> MNNQPQGTNSVPNSIGNIFSNIGTPSFNMAQIPQQLYQSLTPQQLQMIQQRHQQLLRSRLQQQQQQQQQTSPPPQTHQSPPPPPQQSQPIANQSATSTPPPPPAPHNLHPQIGQVPLAPAPINLPPQIAQLPLATQQQVLNKLRQQAIAKNNPQVVNAITVAQQQVQRQIEQQKGQQTAQTQLEQQRQLLVQQQQQQQLRNQIQRQQQQQFRHHVQIQQQQQKQQQQQQQHQQQQQQQQQQQQQQQQQQQQQQQQQQQQQQQQQQQQQGQIPQSQQVPQVRSMSGQPPTNVQPTIGQLPQLPKLNLPKYQTIQYDPPETKLPYPTYWSDKKADTDTLLYEQIIQRDKINKYSLIRETNGYDPFSIYGFSNKEYISRLWHTLKYYQDLKNTRMKSITSTSQKIPSASIW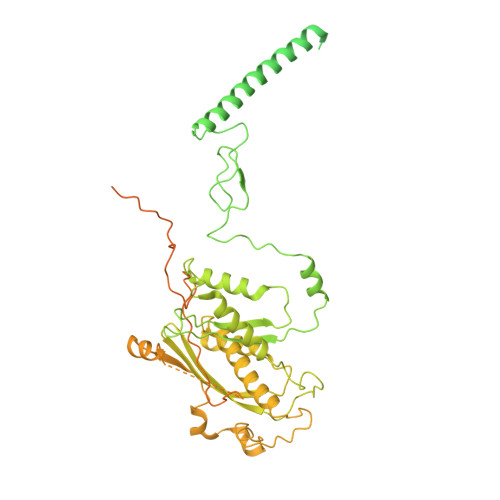GNGYSGYGNGITNTTTRVIPQVEVGNRKHYLEDKLKVYKQAMNETSEQLVPIRLEFDQDRDRFFLRDTLLWNKNDKLIKIEDFVDDMLRDYRFEDATREQHIDTICQSIQEQIQEFQGNPYIELNQDRLGGDDLRIRIKLDIVVGQNQLIDQFEWDISNSDNCPEEFAESMCQELELPGEFVTAIAHSIREQVHMYHKSLALLGYNFDGSAIEDDDIRSRMLPTITLDDVYRPAAESKIFTPNLLQISAAELERLDKDKDRDTRRKRRQGRSNRRGMLALSGTSASNTSMNGVHNTVAAGNASSLPPGEILLPDIADIPRTFRTPVPSTLMPGGVDVGPSVESYELRNTTTYKSRPDRPKPVSPPCYIIDHIPGHSLLLSIKLPGKVNTKEEFAAAPNDTSSGTNAMLPSPESLKTKLNSNIRAGVTIPSIPNPIANHTVTNSPNPTLQPVIPGGAASKSVPTPSLPIAPPVAPHDSEATLLTNSNNGSSNNNTQNTGGSGGDYKDDDDK> MMTMRGLLVGRMQPFHRGHLQVIKSILEEVDELIICIGSAQLSHSIRDPFTAGER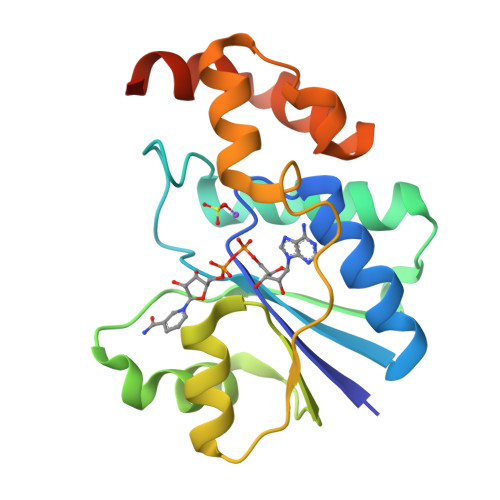VMMLTKALSENGIPASRYYIIPVQDIECNALWVGHIKMLTPPFDRVYSGNPLVQRLFSEDGYEVTAPPLFYRDRYSGTEVRRRMLDDGDWRSLLPESVVEVIDEINGVERIKHLAKKEVSELGGIS> STMALLSQENTQIRDLQQENRELWISLEEHQDALELIMSKYRKQMLQLMVAKK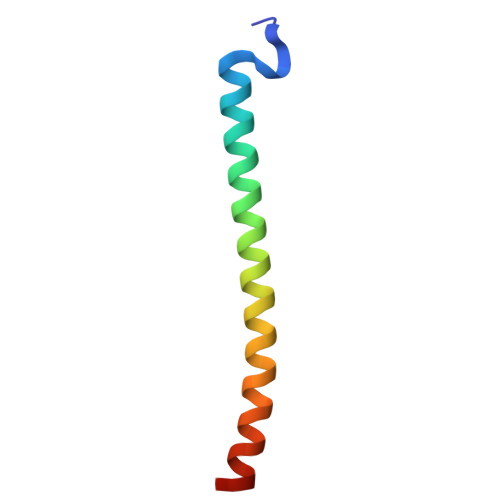A> GMNAIRYTKRECKDEKKITEFLNKARTGFLGLSTNDQPYVIPLNFVWHNHAIYFHGASEGR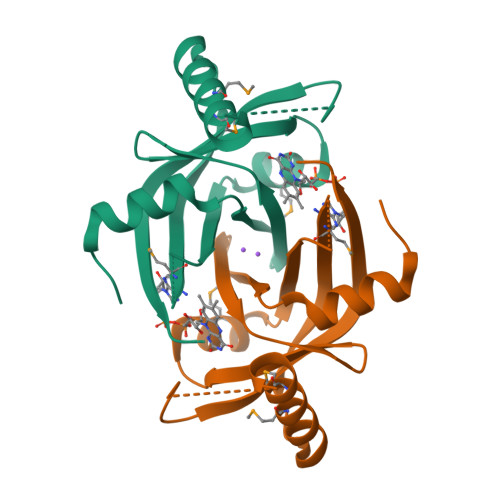KIKMIEANPEVCFTICEDLGTIVSPVPAHTDTAYMSVIIFGTIEPVSAIEEGTEAMQQMLDKYVPGYYHSPLAASHVEKYRSSLGSRTAIYKISCRERTAKVNEPIESLKFYPGRNVSVDKDSR Here, we describe the structure and function of three novel α-amylases from Cordyceps farinosa (CfAM), Rhizomucor pusillus (RpAM) and Thamnidium elegans (TeAM) with a higher stability and pH-tolerance with the potential to act as novel biocatalysts for various industrial processes. The sequence of all three enzymes groups them in the GH13 sub-family 1 along with, for example, the amylase from Aspergillus oryzae (also known as TAKA amylase). All three amylases have the classical domain structure with a central (β/α)8-barrel with the active site located on its C-terminal face, together with a small subdomain, inserted between the third strand and helix and a C-terminal β-sandwich. All three amylases have as their hallmark a shortened loop between β2/α3 and two shorter loops in subdomain B located between β3 and α4 of the central (β/α)8-barrel, compared to structures of other fungal amylases, e.g., TAKA-amylase.

The model of TeAM contains one monomer in the asymmetric unit including residues 1 to 438. Whereas TeAM has no significant activity above pH 7, RpAM and CfAM retain significant activity at pH 7 extending up to a pH of 9. RpAM and TeAM both show a pronounced shoulder, suggesting the involvement of more titratable residues in the substrate recognition and catalysis process. Compared to TAKA amylase, all three amylases show a tendency to produce higher amounts of oligomers with a degree of polymerization (dp) of three, with trace amounts of oligomers with a dp of up to seven for TeAM. Although all three amylases were co-crystallized with acarbose, a well-known inhibitor for amylases, a complex with acarbose bound was only obtained for TeAM and CfAM. As expected, the acarbose was found in the substrate binding cleft in each monomer of TeAM and CfAM, with the acarviosine unit sitting in subsites -1 and +1. The catalytic nucleophile D190/D192(CfAM/TeAM) is in a near attack conformation poised to react with the anomeric carbon, whilst the catalytic acid/base E214/E216(CfAM/TeAM) forms a hydrogen bond with the bridging nitrogen of the glycosidic bond with the 4-deoxyglucose in subsite +1. The +3 subsite is formed by the sugar tong, composed of Y142/144 of subdomain B and F216/218 of the central domain, sandwiching the glucose between them. There are three N-glycosylation sites, one at N144 in RpAM and two at N180 and 412 in TeAM. In the case of TeAM, this is due to the deglycosylation procedure with EndoH.

> AAAADWKSRSIYQLVTDRFGRSDGSTSACGDLSNYCGGDYKGIQNQLDYIAGMGFDAIWISPIPENTDGGYHGYWAKDFEKLNTNFGSADDLKALVTAAHGKGMYVMLDVVANHAGPASGGDYSGFTFSSASNYHPQCTIDYDNQTSVEQCWVADDLPDINTEDDTIVSKLHSIVSDWVTTYDFDGIRIDTVKHIRKDFWSGYEEAAGVFATGEVFDGDAAYVGPYQDQLSSLINYPLYYAIRDVFSAGSGFSRISDMLSTIKSNFKDPSVLTTFVDNQDNARFLSVKSDMSLYKNALAFTILTEGIPVVYYGTEQGFKGGDDPKNREVLWTSNYDTSSDLYKFIKIVNNDVRQKSDKTVTLDVDVGTNTYAFTHGKNLIVVNNYGSGSTESVTVKVGDSVADGTKLVDAVSNITATVSGGSITFSLKDGLPALFVPSS> MDSPLQSTLSSAASPSQAYETYIENGLICLKHKIRNIEKKKLKLEDYKDRLKSGEHLNPDQLEAVEKYEEVLHNLEFAKELQKTFSG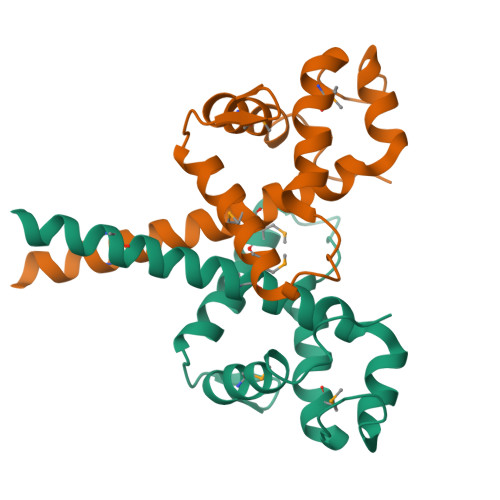LSLDLLKAQKKAQRREHMLKLEAEKKKLRTMLQVQYVLQNLTQEHVQKDFKGGLNGAVYLPSKEMDYLIKFSKLTCPERNESLSVEDQMEQSSLYFWDLLEGSEKAVVGTTYKHMKDLLSKLLNSGYFESIPVPKNAKEKEVPLEEEMLIQSEKKTQLSKTESVKLEHHHHHH>GTTGGGGTTGGGGTTGGGGTTGGG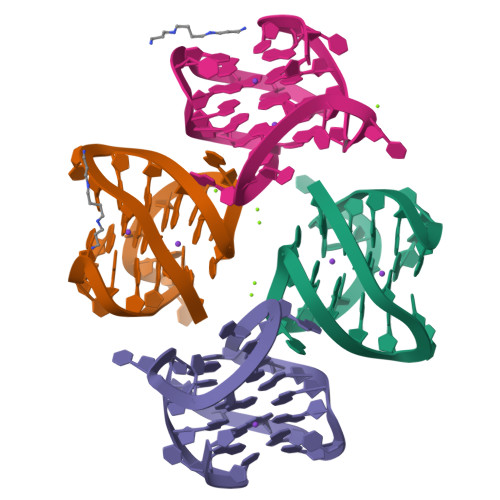G[4x]> GYQDPARSVRHIAIPAHRGLITDRNGEPLAVSTPVTTLWANPKELMTAKERWPQLAAALGQDTKLFADRIEQNAEREFIYLVRGLTPEQGEGVIALKVPGVYSIEEFRRFYPAGEVVAHAVGFTDVDDRGREGIELAFDEWLAGVPGKRQVLKDRRGRVIKDVQVTKNAKPGKTLALSIDLRLQYLAHRELRNALLENGAKAGSLVIMDVKTGEILAMTNQPTYNPNNRR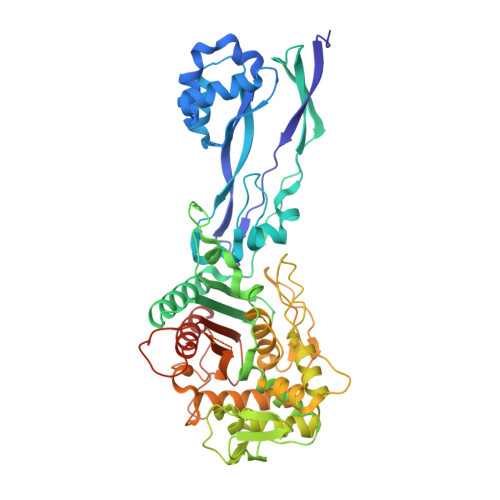NLQPAAMRNRAMIDVFEPGSTVKPFSMSAALASGRWKPSDIVDVYPGTLQIGRYTIRDVSRNSRQLDLTGILIKSSNVGISKIAFDIGAESIYSVMQQVGLGQDTGLGFPGERVGNLPNHRKWPKAETATLAYGYGLSVTAIQLAHAYAALANDGKSVPLSMTRVDRVPDGVQVISPEVASTVQGMLQQVVEAQGGVFRAQVPGYHAAGKSGTARKVSVGTKGYRENAYRSLFAGFAPATDPRIAMVVVIDEPSKAGYFGGLVSAPVFSKVMAGALRLMNVPPDNLPTATEQQQVNAAPAKGGRG>[3x]MGTHMYSEQGINNT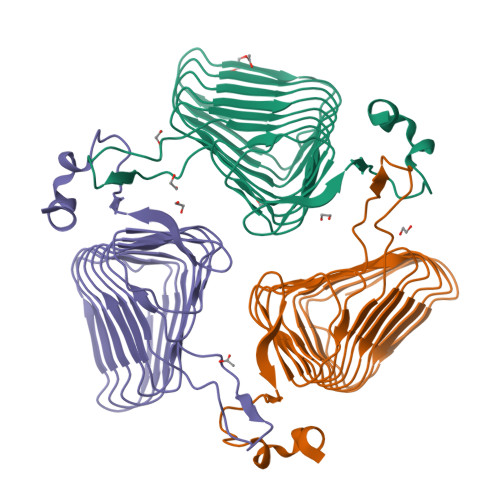INISTTSLTNATQLTVIGNNNSVYIGNNCKIVSSNIRLKGNNITLFIADDVEIMGLVCSLHSDCSLQIQAKTTMGNGEITIAEKGKISIGKDCMLAHGYEIRNTDMHPIYSLENGERINHGKDVIIGNHVWLGRNVTILKGVCIPNNVVVGSHTVLYKSFKEPNCVIAGSPAKIVKENIVWGRKMYHSTMYDDPTLNEFYK>[4x]MAHHHHHHMPGSELISGGWFREENDQWPGQAMSLRVEKVLYDAPTK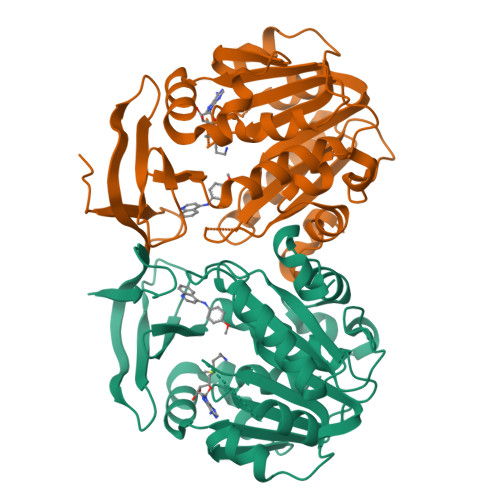FQHLTIFESDPKGPWGTVMALDGCIQVTDYDEFVYHEVLGHTSLCSHPKPERVLIIGGGDGGVLREVLRHGTVEHCDLVDIDGEVMEQSKQHFPQISRSLADPRATVRVGDGLAFVRQTPDNTYDVVIIDTTDPAGPASKLFGEAFYKDVLRILKPDGICCNQGESIWLDLELIEKMSRFIRETGFASVQYALMHVPTYPCGSIGTLVCSKKAGVDVTKPLRPVEDMPFAKDLKYYDSEMHKASFALPRFARHINNSE>[3x]AHNNENVSGISAYLLGLIIGDGGLYKLKYKGNRSEYRVVITQKSENLIKQHI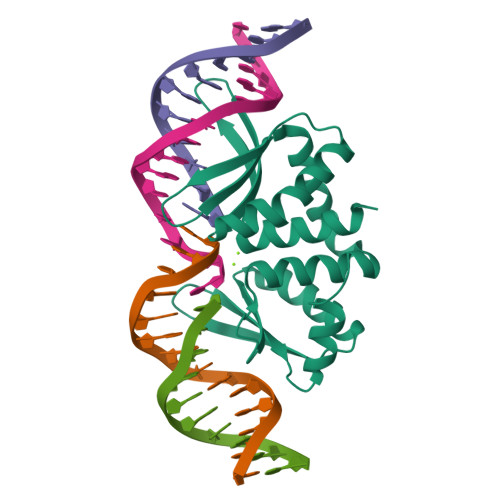APLMQFLIDELNVKSKIQIVKGDTRYELRVSSKKLYYYFANMLERIRLFNMREQIAFIKGLYVAEGDKTLKRLRIWNKNKALLEIVSRWLNNLGVRNTIHLDDHRHGVYVLNISLRDRIKFVHTILSSHLNPLPPEAAALEHHHHHH> QQP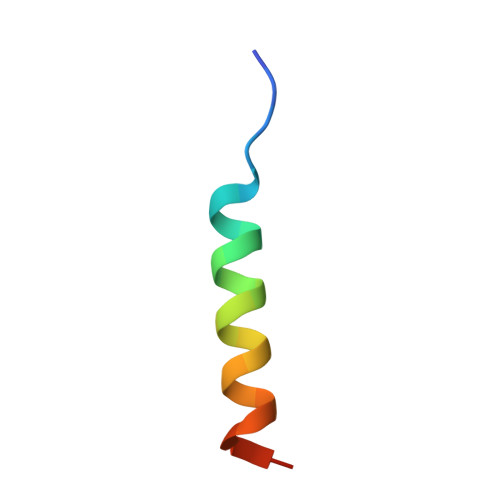TYVALSYINRFMTDAARREQES> MNTNNIKKYAPQARNDFRDAVIQKLTTLGIAADKKGNLQIAEAETIGETVRYGQFDYPLSTLPRRERLVKRAREQGFEVLVEHCAYTWFNRLCAIRYMELHGYLDHGFRMLSHPETPTAFEVLDHVPEVAEALLPESKAQLVEMKLSGNQDEALYRELLLGQCHALHHAMPFLFEAVDDEAELLLPDNLTRTDSILRGLVDDIPEEDWEQVEVIGWLYQFYISEKKDAVIGKVVKSEDIPAATQLFTPNWIVQYLVQNSVGRQWLQTYPDSPLKDKMEYYIEPAEQTPEVQAQLAAITPASIEPESIKVLDPACGSGHILTEAYNVLKAIYEERGYRTRDIPQLILENNIFGLDIDDRAAQLSGFAMLMLARQDDRRILGRGVRLNIVSLQESKLDIAEVWTKLNF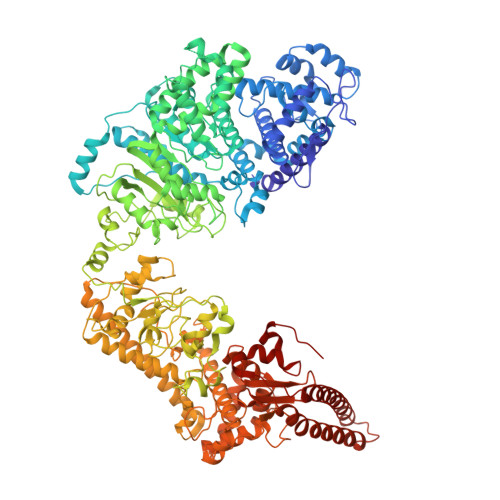HQHMQRGSMGDMFTQGTALANTDSAEYKLLMRTLALFTSAKTLGSLIQVPQEDEAALKAFLEGLYRLAVEGDIQQKEAAAELIPYIQQAWILAQRYDAVVANPPYMGGKGMNGDLKEFAKKQFPDSKSDLFAMFMQHAFSLLKENGFNAQVNMQSWMFLSSYEALRGWLLDNKTFITMAHLGARAFGQISGEVVQTTAWVIKNNHSGFYKPVFFRLVDDNEEHKKNNLLNRMNCFKNTLQNDFKKIPGSPIAYWATLAFINSFLKLPALGTRAVKGLDTNGSIDVFLRRWPEVSINSFDALGKGNSKWFPIAKGGELRKWFGNHEYIINYENDGIELRKNKANLRNKDMYFQEGGTWTVVSTTGFSMRYMPKGFLFDQGGSAVFCENNDELSIYNILACMNSKYINYSASLICPTLNFTTGDVRKFPVIKNNHLEDLAKKAIEISKADWNQFETSWEFSKNKLIEHKGNVAYSYASYCNFQDKLYEQLVNIEKNINNIIEEILGFKIETTENSELITLNSNKIYRYGQSETNDTFLNRHRSDTISELISYSVGCQMGRYSLDREGLVYAHEGNKGFADLVAEGAYKTFPADSDGILPLMDDEWFEDDVTSRVKEFVRTVWGEEHLQENLEFIAESLCLYAIKPKKGESALETIRRYLSTQFWKDHMKMYKKRPIYWLFSSGKEKAFECLVYLHRYNDATLSRMRTEYVVPLLARYQANIDRLNDQLDEASGGEATRLKRERDSLIKKFSELRSYDDRLRHYADMRISIDLDDGVKVNYGKFGDLLADVKAITGNAPEVI>[2x]MTEKKERIDVHAYLAEFDDIPGTRVFTAQRARKGYNLNQFAMSLMKAENRERFKADESAYLDEWNLTPAAKAAVLARDYNAMIDEGGNVYFLSKLFSTDGKSFQFAAGSMTGMTQEEYAQMMIDGGRSPAGVRSIKGGY;>MARVTTGITSSHIPALGAAIQTGTSDNDYWGPVFKGYQPIRDWIKQPGNMPDVVILVYNDHASAFDMNIIPTFAIGC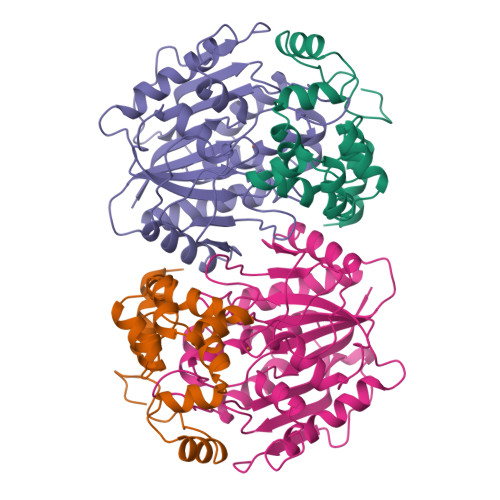AETFKPADEGWGPRPVPDVKGHPDLAWHIAQSLILDEFDMTIMNQMDVDHGCTVPLSMIFGEPEEWPCKVIPFPVNVVTYPPPSGKRCFALGDSIRAAVESFPEDLNVHVWGTGGMSHQLQGPRAGLINKEFDLNFIDKLISDPEELSKMPHIQYLRESGSEGVELVMWLIMRGALPEKVRDLYTFYHIPASNTALGAMILQPEETAGTPLEPRKVMSGHSLAQA[2x]>[4x]SMRRIVVTGMGMINSLGLNKEDSFLAIAKGECGIKHIESFDASAFPVRIAGEITDFDPTEVMNPKDVKKAGRFIQLALKATREAMKDSGILDAHNRCPEELANRMGVSSGSGIGGLGNIEANSIFCFEKGPRKVNPFFITSALVN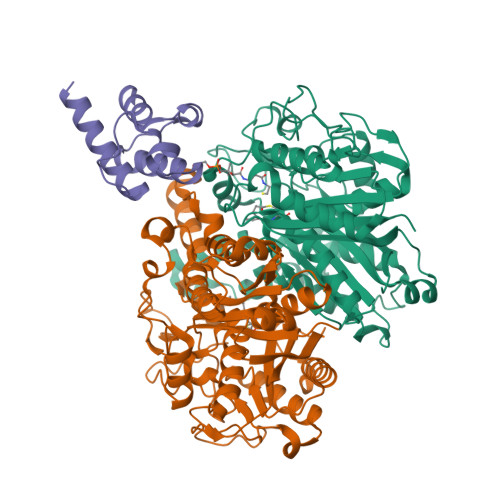MIGGFTSIEFGIKGPNLSSVTACAAGTHAIIEAVKTILLNGADRMLVVGAESTICPVGIGGFASIKALSTRNDEPKKASRPFDKDRNGFVMGEGAGALVLEEYESAKKRGAKIYAEFAGYGESGDANHITAPAPEGEGAFRAMKMALEMAKVEVGYVNAHGTSTHYNDLYESIALKNVFGSKEKVPPVSSTAGQIGHCLGAAGALEAVISIMAMNQGILPPTINQETPDPECDLDYIPNAAREKQVDAVMSNSFGFGGTNGVVIFKKA;>[2x]GTSSMGYLMALFEDIQAVIAEQLNVDAAQVTPEAEFVKDLGADSLDVVELIMALEEKFGIEIPDEQAEKIVNVGDVVKYIEDNKLA(1R,3R)-5-[(2E)-2-[(1R,3aS,7aR)-1-[(2R,3S)-3-ethyl-5-oxidanyl-pentan-2-yl]-7a-methyl-2,3,3a,5,6,7-hexahydro-1H-inden-4-ylidene]ethylidene]-2-methylidene-cyclohexane-1,3-diol 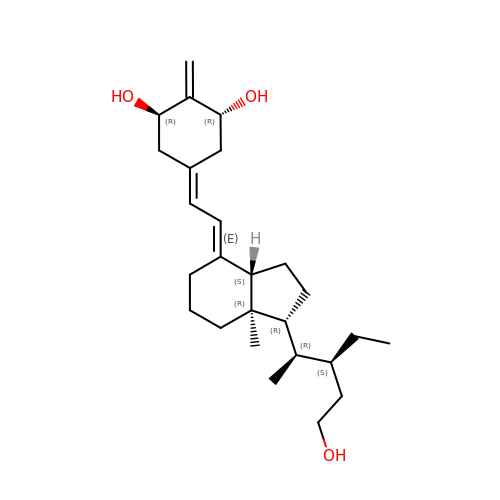| C26 H42 O3 | MJSNOTROAGEHAK-HSPXBGPKSA-N>VGAIMLDGKATRDEIFGDLKQRVAALDAAGRTPGLGTILVGDDPGSQAYVRGKHADCAKVGITSIRRDLPADISTATLNETIDELNANPDCTGYIVQLPLPKHLDENAALERVDPAKDADGLHPTNLGRLVLGTPAPLPCTPRGIVHLLRRYDISIAGAHVVVIGRGVTVGRPLGLLLTR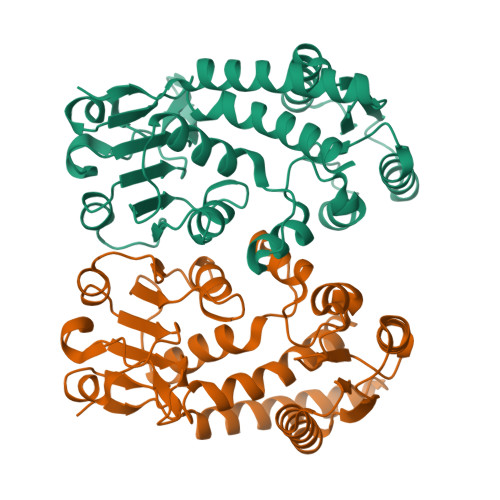RSENATVTLCHTGTRDLPALTRQADIVVAAVGVAHLLTADMVRPGAAVIDVGVSRTDDGLVGDVHPDVWELAGHVSPNPGGVGPLTRAFLLTNVVELAERR[2x]[[[[(2R,5S)-5-(4-azanyl-5-fluoranyl-2-oxidanylidene-pyrimidin-1-yl)-1,3-oxathiolan-2-yl]methoxy-oxidanyl-phosphoryl]oxy-oxidanyl-phosphoryl]amino]phosphonic acid | C8 H14 F N4 O11 P3 S | 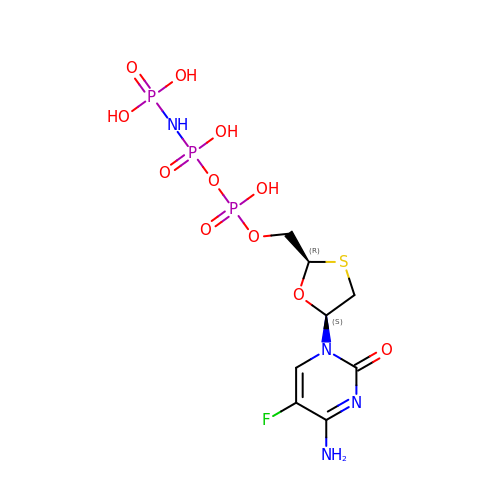LBSQECIRXSOKHJ-NTSWFWBYSA-N> MFVW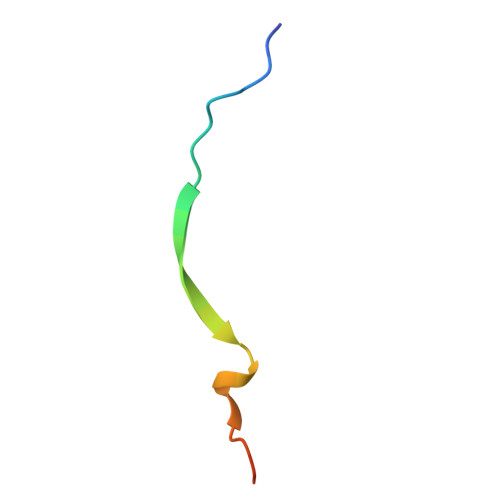TNVEPRSVAVFPWHSLVPFLAPSQ> SNAGSINGVPLLEVDLDSFEDKPWRKPGADLSDYFNYGFNEDTWKAYCEKQKR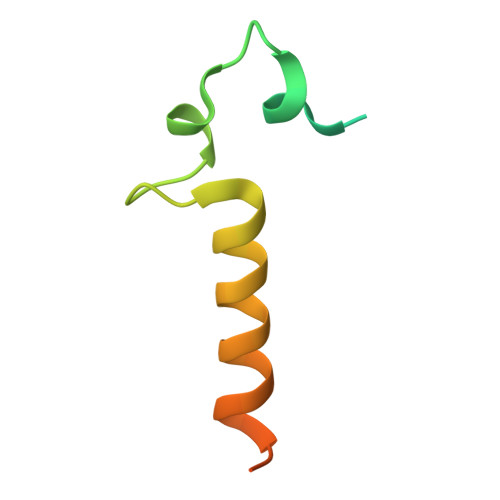IRMGLEVIPVTSTTNK>[3x]UUUUUAAUG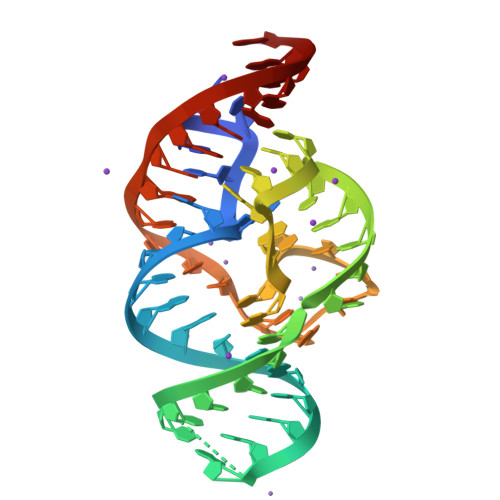AAGCCACAGGCCUGUGAGGGUCCUAAGCCCCUAAUUCAGAAGGGAAA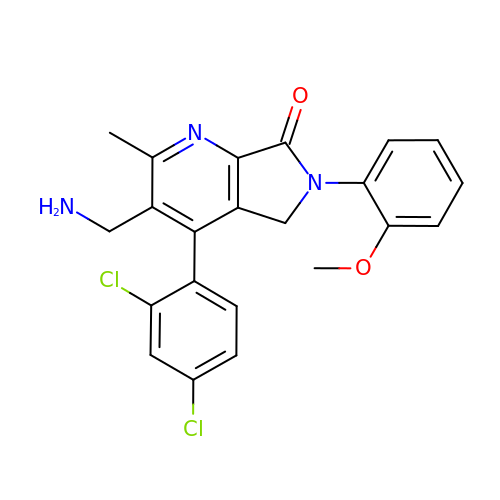3-(aminomethyl)-4-(2,4-dichlorophenyl)-6-(2-methoxyphenyl)-2-methyl-5,6-dihydro-7H-pyrrolo[3,4-b]pyridin-7-one | C22 H19 Cl2 N3 O2 | YFKUZVBMNGNFRI-UHFFFAOYSA-N Singapore grouper iridovirus (SGIV), one of the nucleocytoviricota viruses (NCVs), is a highly pathogenic iridovirid. Here, we report the cryo-EM structure of the SGIV capsid at 3.5 Å resolution using a block-based reconstruction method. The cryo-EM map, combined with viral proteomics, crosslinking mass spectrometry (CXMS) and fluorescence colocalization assays, enables us to identify the major capsid protein (MCP) and seven types of minor capsid proteins (mCPs). The atomic models for an asymmetric unit (ASU) of the viral capsid constituted by different copies of these capsid proteins are further determined.

In one ASU, there are 41 MCP capsomers, of which six are in the pentasymmetron, and the other 35 are in the trisymmetron. Similar to PBCV-137, the structural alignment analysis revealed that the N-terminal residues of the SGIV MCPs are conformationally diverse and can be grouped into three configurations (NI, NII and NIII). NI displays a hook-like shape, NII is perpendicular to the capsid surface, and NIII is parallel to the bottom of the capsid. Based on the information from the cryo-EM map and proteomics of the purified SGIV sample, the penton protein was ultimately determined to correspond to the VP14 protein, which is a polypeptide encoded by the orf14 gene and harbors eight potential β-strands. Each VP14 protomer contacts two MCP protomers from two adjacent pseudo-hexameric capsomers. However, the AA sequences and structures of these zip proteins have not been identified except for that of PBCV-137. Using the method described above for the SGIV penton protein, the SGIV zip protein was identified as the VP38 protein encoded by the orf38 gene. The atomic model of VP38 (P1) shows that two VP38 protomers are interlocked into a dimer, which may contribute to gluing two antiparallel MCP capsomers together. The space generated by these missing residues is occupied by another mCP (P2) VP139. The TmP (P3) of SGIV corresponds to the VP137 protein encoded by the orf137 gene. VP88, encoded by the orf88 gene, was identified as the anchor protein (P5) of SGIV.

>[123x]MTCTTGAGVTSGFIDLATYDNLDRALYGGKDATTYFIKEHYPVGWFTKLPTMATRVSGNPAFGQEFSVGVPRSGDYVLNAWLTLKTPEIKLLETNRLGANGTVRWTKNLMHNAVEHASLTFNDICAQQFNTAYLDAWTQFNMCEGKRIGYDNMIGNTSDMTNPTPAQGQDGARTLPSKNLVLPLPFFFSRDCGLALPTVVLPYNEIRINIKLRSLQELLVFQNKDTGNVIPISATDIAGGLADTVEAYVYMTVGLVSNVERCAMAGTVRDMVVEQMQAAPTHIVNPQNTNNVHVDMRFSHAVKALFFMVQNVTYKSVGSNYTCVTPVNGPGNTVMEPAMSVDPIKSASLTYENTTRLANMGVEYYSLVQPWYFSASIPVYTGYHMYSYALNVGSVHPSGSTNYGRLTNASITVTMSPESVVAAAGGGNNNSGYNEPQRFALVVIAVNHNVIRIMNGSMGFPIL;>[15x]MIHNYAILIVTAAVVVWYYYKLYVVDKNGKKSLVRTRKHRNLESAARRDPILKTYSKQDGTRSRKPKSTKKEPHWMDPQLMGSQTTQYSRNRGYGDPIRGDLPIVPDDGGWFATRANPAHHLHTGALSMIGGDASDCGSTAVQQLIKKYEDKGCNNNGLNVMSSHYGGVM;>MDCATYATRKDKGWELNENRCVWAASVKPTSGAIMTNVGVHGKSGNAVLMTPKRRPHAQNHAGYKIKYCKQVPLIPLHGGDYILNHWETRGVDRMRIPGIQHAPPPPAPSGMQNAYSTHPDAYRTPLLADSHALSRMPVVQVHGPQVAPKNSHFTVAPEKHGPVEDMNAIINALPTKVDAVKLEYSASKTNRTNKRPGDGGAPPPKNLSKCHQNKLKTFARTANSGANPFRPATAAPQGLSKQPVRKPFASARNANSGANPFRPPLAHQGLSKAHVVKTAVSVANRSAGAEPFVTRNDPRALAMELANNKTISVTLGLRHWKTVSAAPPEKMSKSGVCKIATNVYNRDGGANPFLVKYEPDSLAVCPMETVEIAAVPSKRPWEGSANPRRPEQISFGMSDKPKFVNDKIGIVLRGPTLAPTLDRTATHTVTRPRALGSFHSTAGPAKHAASIMAECKDESR[2x];> MYRGFSLKLPNNYRSGQVTTEHRLPASNSHARWPVEVSFYSAVLHVPAKHQHKFPPVLELKLHNMTTGSMAAHRGSGHHFTFMFHAQSSPTEAVYSCVPVPIVFSDYQSNVIASVDMGEHDTAEKLHFYGSIRNCDNGCTY;> MGAAQSVNGVKIVTNAYAEIMTDLAVDQDITADQTQVFSIDNVSGDVYVEGTVMTEKLVINLASLMKAVTNQSSQDELIDNIAQQAQAAVSGLNFAQFAFVTNNIDRLITACVKLSVDMRVSCTAKVEMTQSFSVSSVMGDVRVKDVRMEEFSDVISTCALNAAITNAQLSDIVSQIKQRGDATATGLNPMAILAAVVLAIIGLPLGAGFLAGRRVVGPLMMVTGMVGGGALAMGYVPEPIKLTGFAPEPDLTAVVPVAVENGLTLKAAISKLTGDPQYGAVYWQNYKVTGTTAVKLNQTVSYYAPPNFDPVTWTASEPAQKQPSFRVFPTLFQGQGLPKISYRLAYGTVALTQGPERGDVYLDSTTGNYYVLKDGWKLNGTIPGAIKDRPEAWGIVDPNETTALTGSERYTWVDPYTRVQGTLWYKPKDSHEWVKERQDPVPINVPLTETPSDFNVWVYKDATAKKIVGWVSAGAGAAGAGLTASAYFMPSTAVDAKAEVGEAAK;> MDSQGFWAILAFTPVLMILSLKGEGLLAMVGLLVLTVTLLASREKNDRPRLSCRGKIGRKVSGFENAGHVRDSHHVIYKRPPVNEYCAETREDNSLYVPEYCGQNWKNGVLSGMGTHHDAYRNLAVNMMTLRRESAVSAGWAHSYL;> MNAYQNDKLHLCAPRPDLVRAAMSAMVRETGCTPNVNIREMAISAGVMLTKIRANPGMLRYGMTATQTVIYNLKELFAAHAARGVVFKTPAIHPAHPSQWKGF> MSMMAERDMGRILLDLSDDVIQRLDDL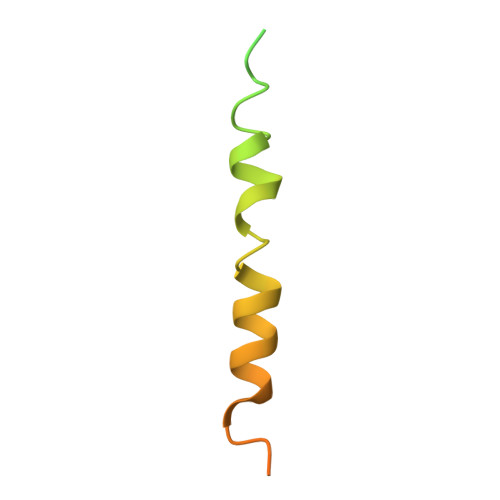KVQRNIPRAELLREAVEQYLEKQDRAKDTISSALGLWQDCEEDGMEYQRQLRKEW>[2x]SILRVDANRIDYLLNLV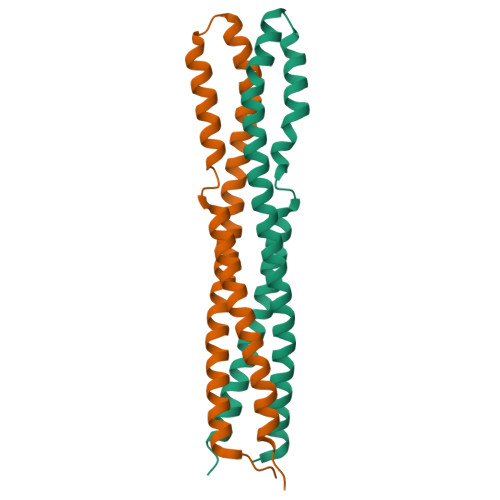SETVITKASLNQSTIEFAELYDKFQNSSTIYKDKTRRLLDKMPEYLEKIQQGYDINSIKQDVLNEYSSLLEVFGDFDSLMKAAVTKFKSSSQNLGRISGELQEGVMKIRMVP>[4x]MPSIKPPLIAVELENPMLGEVIDLEETKAIVIAAYENKALALLFDYYTGEIKQINRQGNTYKIAVSEDYIGGIFNGFGEPIKGPKPYPEDYRDINGLAINPYARKVPNEILYTGISS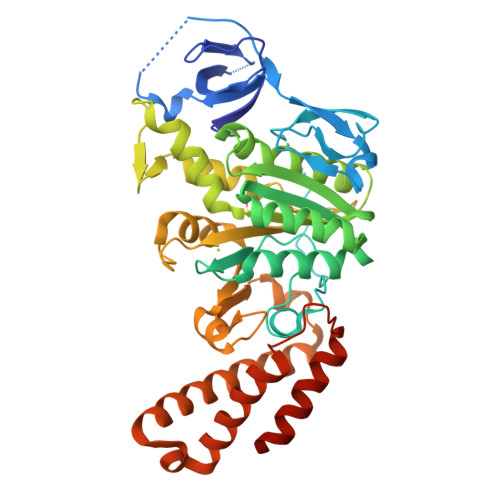IDVAHPLLKGQKIAIFSPPGLPMERLALQIARNVAKDKTIIFAAIGVPSDIYKMFIDEFINTKAIMNSAIFISKADSSPIEKIYTPRVALTLAEYLAFEKNRDVLVLMLDMTNYADALREISTLRKEIPSRRGYPAYLYTDLASIYERSGLTSKGSITLIPMLTMPGNDITHVVPDLTGYITEGQYVLSQDLHSKNIYPPIDLLKSLSRLAKNGMSKKHKKYADILIKSYAKGLEARDIATIVGEDSLSKEDKAYLKFAELVEKEFIKQDYYEYRSIEKSFEIIDSILSQSGLPYSPIQ> MT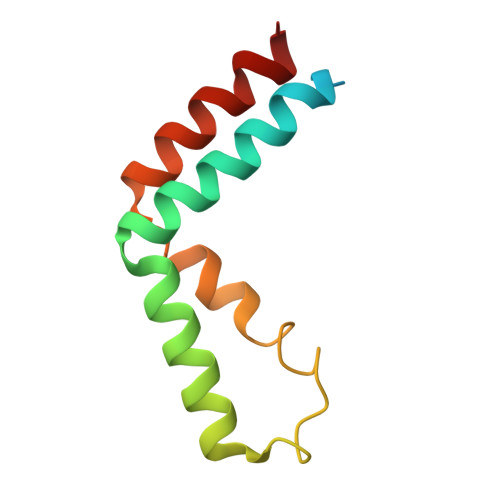INKETGTDPDPGYKPTLRSQDKAALKELLHTRLVECGWHKDIKEMIRNIIMERGVDNINRDQLAAQIVPQARALVPEVVKNEMMLRVHAALDK A3H is the most polymorphic member of the APOBEC family, as its mRNA can undergo alternative splicing to generate four splicing variants (SVs), and has seven distinct human A3H haplotypes (hap I-VII) containing various combinations of five single nucleotide polymorphisms. Literature suggests that the anti-HIV activity of A3H can be through both deaminase dependent and independent manners, and the different anti-HIV activities of the A3H variants were attributed to a combination of different factors, such as differences in RNA binding and virion packaging, protein stability, deaminase activity, and subcellular localization. Evidence so far suggests that binding to RNA is largely responsible for the multimerization of A3H and some other APOBEC members. RNase A treatment is required to activate or enhance the deamination on ssDNA for A3H and several APOBEC members, which suggests overlapping binding sites for both RNA and ssDNA substrates.

While A3H m1 carries a set of 7 mutations and produced a stable dimer form, stable monomeric forms can be isolated from both A3H m1+H114A and m1+W115A/C116S mutants. With these stable dimeric and monomeric forms of the A3H WT and mutants in hand, we performed crystallization trials either with the MBP tag or the cleaved forms, with or without nucleic acids, and obtained a high-quality crystal form of the cleaved A3H m1+W115A/C116S monomer that diffracted to 2.49 Å resolution. The A3H m1+W115A/C116S monomeric structure was determined to 2.49Å resolution and refined to excellent statistics. Each asymmetric unit (asu) contains two A3H molecules that have nearly identical structure for the core fold and the loops. Notably, helix 6 (h6) of A3H extended six amino acid residues (1.7 turns) at its N-terminal side, making it the longest h6 among all APOBECs. The canonical short beta strand 5 (β5) of APOBEC proteins is not a typical strand in this A3H monomeric structure. The disruption of β5 appears to result from the proline residue (P132) that forms an outward-facing bulge and moves away from β4, disrupting the already short β5, which may reflect an alternative conformation of β5 in A3H natural state. In addition to β5 strand, the A3H monomer contains a long loop 1 around the Zn-center. The monomeric structure also shows that A3H is highly positively charged on one end around the Zn-active center, and more or less neutral and negatively charged on the other end. In addition, stable monomeric A3H can be obtained simply by mutating H114 or W115/C116 (as mutants A3H m1+H114A and m1+W115A/C116S), suggesting that H114 and W115 participate in nucleic acid binding and their interactions with RNA are critical for dimer formation.

>[2x]ALLTAETFRLQFNNKRRLRRPYYPRKALLCYQLTPQNGSTPTRGYFENKKKCHAAICFINEIKSMGLDETQCYQVTCYLTWSPCSSCASELVDFIKAHDHLNLRIFASRLYYHASKPQQDGLRLLSQEGVPVEVMGFPEFADCWENFVDHEKPASFNPYKMLEELDKNSRAIKRRLDRIKS>[2x]MAEELKRSIPLLPLRGLLVYPTMVLHLDVGRDKSVQALEQAMMHDHMIFLAT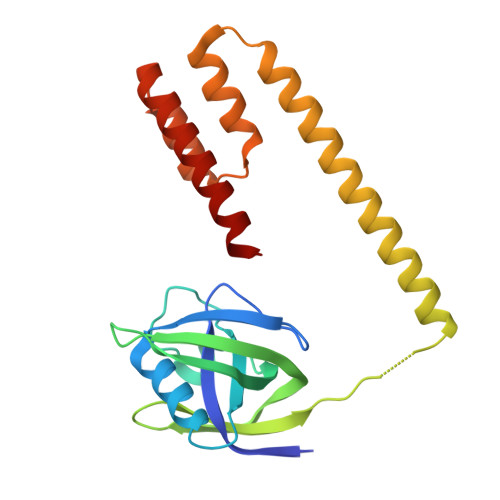QQDISIDEPGEDEIFTVGTYTKIKQMLKLPNGTIRVLVEGLKRAHIVKYNEHEDYTSVDIQLIHEDDSKDTEDEALMRTLLDHFDQYIKISKKISAETYAAVTDIEEPGRMADIVASHLPLKLKDKQDILETADVKDRLNKVIDFINNEKEVLEIEK>GRKKIQITRIMDERNRQVTFTKRKFGLMKKAYELSVLCDCEIALIIFNSSNKLFQYASTDMDKVLLKYTEYNEPHESRTN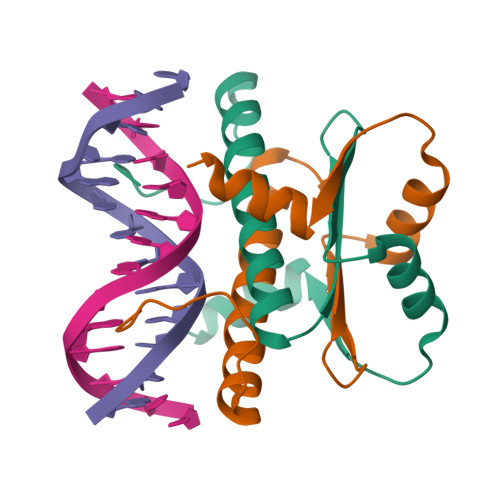SDIVEALNKK[4x]> MDVHIDNQVLSGLGTPLLVHLFVPDTVMAELCPNRVPNCEGAWCQTLFSDRTGLTRVCRVFAARGMLPGRPSHRGTFTSVPVYCDEGLPELYNPFHVAALRFYDEGGLVGELQIYYLSLFEGAKRALTDGHLIREASGVQESAAAMQPIPIDPGPPGGAGIEHMPVAAAQVEHPKTYDLKQILLEITQEENRGEQRLGHAGSPALCLGLRLRAGAETKAAAETSVSKHHPALENPSNIRGSAGGEGGGGRAGTGGTVGVGSGALSRVPVSFSKTRRAIRESRALVRGIAHIFSPHALYVVTYPELSAQGRLHRMTAVTHASPATDLAEVSILGAPEREFRFLISVALRISASFREKLAMQAWTAQQEIPVVIPTSYSRIYKNSDLIREAFFTVQTRVSWESCWVKATISNAPKTPDACLWIDSHPLYEEGASAWGKVIDSRPPGGLVGAASQLVALGTDGHCVHLATTSDGQAFLVLPGGFVIKGQL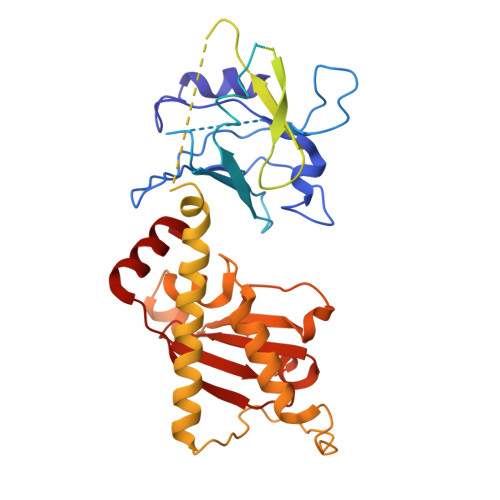ALTPEERGYILARHGIRREQ> MCFSPKIKTPKMDTNQIRAVEPAPLTQEVSSVEFGGS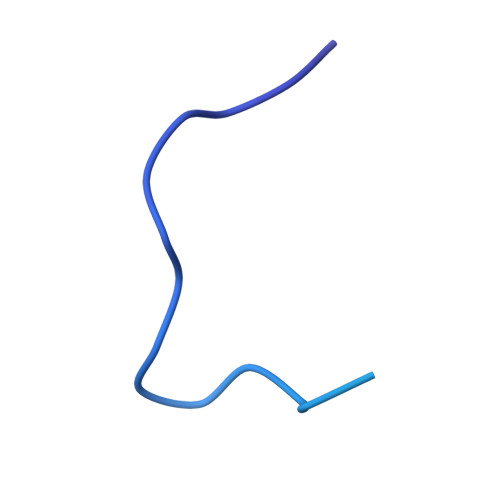SDETDTEGTEVSGRKGLKVERDDSVAKSKASGNGSARMKSSIRKSAFGGKK>[2x]XMDKLREKINAARAETDEAVARAEAAEAKLKEVELQLSLKEQEYESLSRKSEAAESQLE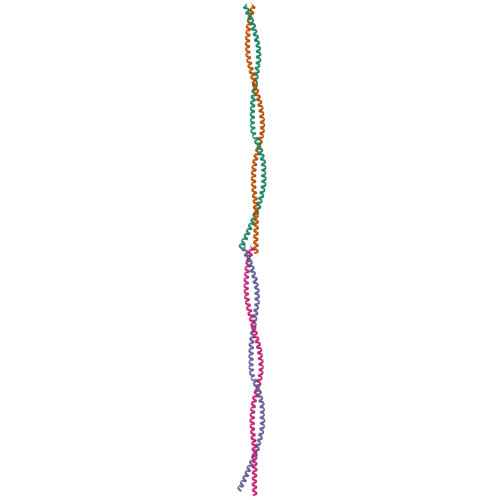ELEEETKQLRLKADNEDIQKTEAEQLSRKVELLEEELETNDKLLRETTEKMRQTDVKAEHFERRVQSLERERDDMEQKLEEMTDKYTKVKAELDEVHQALEDL6-[(1S)-1-(azepan-1-yl)ethyl]-N,N-dimethyl-1,3,5-triazine-2,4-diamine | C13 H24 N6 | 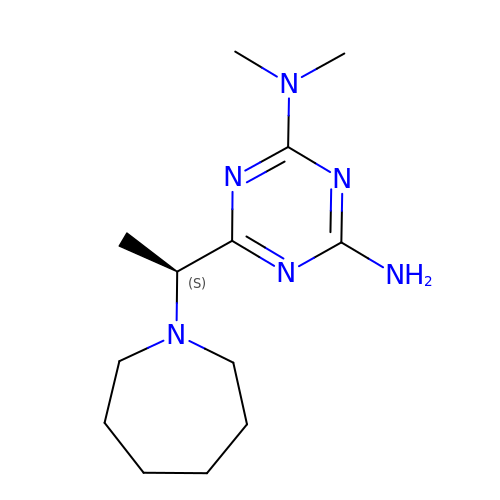VXAHGJQOHMSESG-JTQLQIEISA-N> MPLHMIPQVAHAMVRAAAAGRLTLYTRTRTETTNFDHAEYVTCGRYTICAFCLTTLAPHANVKTIQDSHACSRQPNEAIRSLVEVSDKAQTALVGSRTVDYHELDVKAGFVAPTADETIAPSKDIVELPFRTCDLDDSSATACVRNHCQAGHDGVIHLPILSGDFKLPNEHPTKPLDDTHPHDKVLTRCPKTGLLLVHDTHAHAT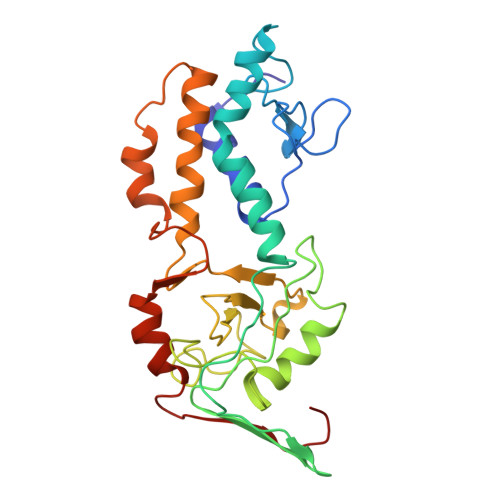AVVATAATRAILMHDLLTSANADDGHQARSACYGPAFNNLTFACHSTCASDMAHFDCGQIVGLDLHVEPSD> MAATRQIQYTIPPREDYNKLSDEQKTRISEAFELFDSNKDGLLSYEEFRFVLRALGFDLPKQQTYDMLVRHGQRPANWPHDQECPPVYRQFNLATAQALAGTLIRQRDPRDELRRAFRLFDVDGKGMITEDDLRK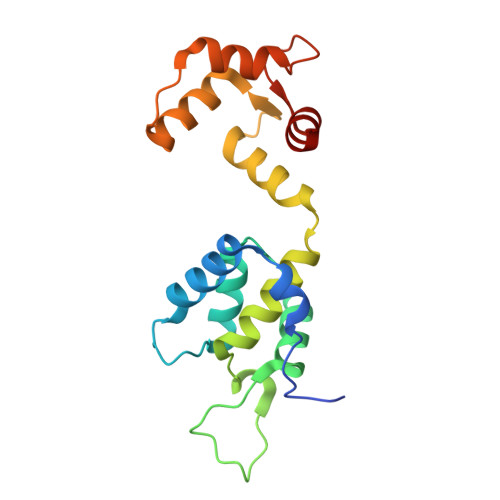VCQQVGNNIPDADIQAMIEEFDSNGKGGVDEDEFLRLMMSKK> ACSFPKCPWVEGCAX;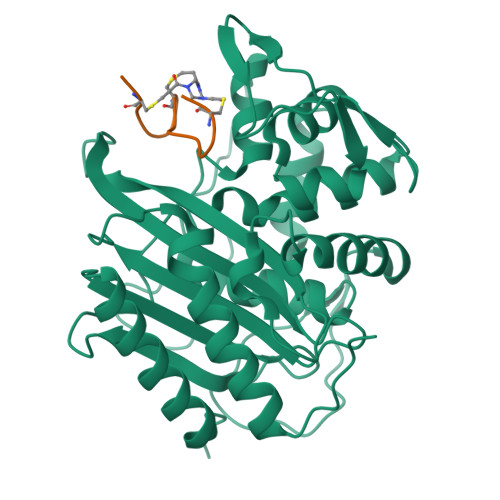> GPGYQDPLSIDERLQALVYRELNNAVAFNKAESGSAVLVDVNTGEVLAMANSPGRNRTITDVFEPGSTVKPMVVMTALQRGVVRENSVLNTIPYRINGHEIKDVARYSELTLTGVLQKSSNVGVSKLALAMPSSALVDTYSRFGLGKATNLGLVGERSGLYPQKQRWSDIERATFSFGYGLMVTPLQLARVYATIGSYGIYRPLSITKVDPPVPGERVFPESIVRTVVHMMESVALPGGGGVKAAIKGYRIAIKTGTAKKVGPDGRYINKYIAYTAGVAPASQPRFALVVVINDPQAGKYYGGAVSAPVFGAIMGGVLRTMNIEPDALTTGDKNEFVINQGEGTGGRS OATP1B1, encoded by SLCO1B1 and formerly known as SLC21A6, LST-1, OATP-C, or OATP2, is specifically expressed on the basolateral membrane of hepatocytes. OATP1B1 plays a vital role in mediating the uptake of endogenous compounds such as bile acids, bilirubin, steroid conjugates, and thyroid hormones, as well as a large variety of clinical drugs including statins, antibiotics, antivirals, and anticancer medications for hepatic clearance. The overall architecture of OATP1B1 is composed of the transmembrane domain (TMD) and extracellular loops (ELs) with both N- and C-terminal ends situated in the cytoplasm. The interface between NTD and CTD of OATP1B1 forms a conserved cavity in which substrates bind.

Compared to lipophilic estrone and estradiol, the estrogen ester and conjugate, E3S, is unable to permeate through cell membranes and is transported mainly via OATPs, which has been widely used as a prototypical model substrate of OATP1B1.43–45 Inhibitors of OATPs are of interest in treating estrogen-associated cancers. In our study, the cryo-EM structures of OATP1B1–E unexpectedly revealed three different conformations: inward-open state with high resolution, outward-open and occluded states with moderate to low resolutions. After extensive trials, we successfully obtained the inward-open structure of OATP1B1–Ein at a resolution of 3.2 Å, with OATP1B1–Eou and OATP1B1–Eoc resolved at moderate to low resolutions. Densities of E3S were found in all three conformations at similar sites. The EM density of E3S in OATP1B1–Ein is unambiguously resolved, allowing us to discern the pose of the E3S with high confidence. The inward-open structure of OATP1B1–Ein opens its central substrate cavity towards the cytoplasm. Like DCF, E3S also binds at the minor pocket, with its sulfate group extending into the interior of the CTD. F356 forms hydrophobic packing with the estrone group of E3S, together with Y352 and F386, enclosing the hydrophobic body of E3S. Additionally, residues from the minor pocket, Y625, Y422, Q541 and N544 form hydrogen-bond interactions with the sulfate group of E3S. Mutagenesis of Q541A exhibited a significantly varied IC50 value for E3S, supporting the essential role of Q541 for the binding of E3S. In the inward-open OATP1B1–Ein, accompanying the disappearance of the intracellular gate, an extracellular gate is generated by electrostatic interactions between NTD and CTD.

> MDQNQHLNKTAEAQPSENKKTRYCNGLKMFLAALSLSFIAKTLGAIIMKSSIIHIERRFEISSSLVGFIDGSFEIGNLLVIVFVSYFGSKLHRPKLIGIGCFIMGIGGVLTALPHFFMGYYRYSKETNINSSENSTSTLSTCLINQILSLNRASPEIVGKGCLKESGSYMWIYVFMGNMLRGIGETPIVPLGLSYIDDFAKEGHSSLYLGILNAIAMIGPIIGFTLGSLFSKMYVDIGYVDLSTIRITPTDSRWVGAWWLNFLVSGLFSIISSIPFFFLPQTPNKPQKERKASLSLHVLETNDEKDQTANLTNQGKNITKNVTGFFQSFKSILTNPLYVMFVLLTLLQVSSYIGAFTYVFKYVEQQYGQPSSKANILLGVITIPIFASGMFLGGYIIKKFKLNTVGIAKFSCFTAVMSLSFYLLYFFILCENKSVAGLTMTYDGNNPVTSHRDVPLSYCNSDCNCDESQWEPVCGNNGITYISPCLAGCKSSSGNKKPIVFYNCSCLEVTGLQNRNYSAHLGECPRDDACTRKFYFFVAIQVLNLFFSALGGTSHVMLIVKIVQPELKSLALGFHSMVIRALGGILAPIYFGALIDTTCIKWSTNNCGTRGSCRTYNSTSFSRVYLGLSSMLRVSSLVLYIILIYAMKKKYQEKDINASENGSVMDEANLESLNKNKHFVPSAGADSETHCLEGSDEVDAGSHHHHHHHHHHGSVEDYKDDDDK> MSEEVVQDAPLENNELNAEIDLQKTIQEEYKLWKQNVPFLYDLVITHALEWPSLTIQWLPDKKTIPGTDYSIQRLILGTHTSGNDQNYLQIASVQLPNFDEDTTEFTPSTIRRAQATGSYTIEISQKIPHDGDVNRARYMPQKPEIIATMGEGGNAYIFDTTCHDALTTGEALPQAVLKGHTAEGFGLCWNPNLPGNLATGAEDQVICLWDVQTQSFTSSETKVISPIAKYHRHT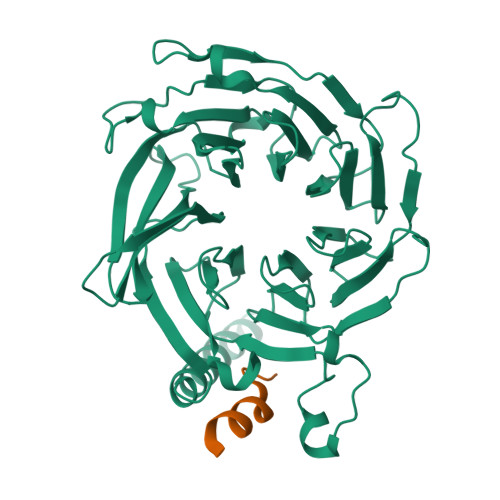DIVNDVQFHPQHEALLASVSDDCTLQIHDTRLNPEEEAPKVIQAHSKAINAVAINPFNDYLLATASADKTVALWDLRNPYQRLHTLEGHEDEVYGLEWSPHDEPILASSSTDRRVCIWDLEKIGEEQTPEDAEDGSPELLFMHGGHTNRISEFSWCPNERWVVGSLADDNILQIWSPSRVIWGRDHVQVSPRDLE;> MDLMPLEKARAIEIAFDNVFHNTKIPDNLQQFDAILKRLERRRFIPTENQKPRVYETELLVLRFREFGVKDNHNHPINLHSLRSKSLIRAQGKKLDLHNRVFLRRNVRAVKM Human CEACAM1 (hCEACAM1) is a single pass type I transmembrane protein expressed as 12 alternatively spliced isoforms that all contain an N-terminal V set fold of the immunoglobulin superfamily (IgV) ectodomain followed by up to three type 2 constant immunoglobulin (IgC2) ectodomains (A1, B, A2), a transmembrane sequence, and a signaling cytoplasmic domain. CEACAM1 function is triggered by intercellular or trans binding of the IgV domain, resulting in higher order surface CEACAM1 oligomerization and subsequent intracellular signal transduction. In contrast to other immunoreceptors such as the T cell inhibitory and mucin domain-containing protein 3 (TIM-3), programmed cell death protein 1 (PD-1), and programmed death-ligand 1 (PD-L1), CEACAM1 serves as its own primary ligand, owing to high affinity homophilic interactions of its unique IgV domain, as well as an important microbial receptor. The displaced CC′ loop forms a cleft with the FG loop that exposes the key residues F29, S32, Y34, V39, G41, Q44, Q89, I91, N97, and E99 critical in mediating homophilic CEACAM1 interactions.

The V39A mutant crystal contained two copies of a hCEACAM1 GFCC′ face–mediated homodimer in the asymmetric unit. The first hCEACAM1 V39A dimer comprising molecules (a) and (b) resembled a WT homodimer with RMSD of 0.7 Å (over 1482 atoms), whereas the second GFCC′-mediated dimer comprising molecules (c) and (d) featured important conformational differences across several beta strands and loops with RMSD of 3.0 Å (over 1655 atoms) compared to the WT homodimer. The major distinguishing feature of this second V39A homodimer structure compared to that of the WT was the increased separation between interacting CC′ loops (10.0 Å vs 3.7 Å). Further, we observed a considerable decrease in hydrogen bond and weaker hydrophobic interactions at the GFCC′ face in the V39A homodimer, consistent with a less stable and less interactive GFCC′ face that possibly reflects an hCEACAM1 IgV monomer–dimer exchange transition state. Interestingly for both of the V39A-containing dimers, a considerable metal ion electron density (4.0 σ intensity in the 2Fo–Fc electron density map) was observed at V39A molecule (a) and (c); the density was modeled as nickel (Ni++) that was hexa-coordinated by residues H105 and V106 from three neighboring IgV molecules found in the unit cell and crystallographic symmetry mates. A CSS of 0.0 was calculated for the weak GFCC′-mediated V39A dimer (formed by molecules (c) and (d)) consistent with a monomeric species whereas a CSS score of 1.0 was calculated for molecules (a) and (b) consistent with a dimer and thus suggestive of the possibility of both hCEACAM1 V39A monomers and dimers and furthermore, a rapid monomer–dimer exchange model.

>QLTTESMPFNVAEGKEVLLLVHNLPQQLFGYSWYKGERADGNRQIVGYAIGTQQATPGPANSGRETIYPNASLLIQNVTQNDTGFYTLQVIKSDLVNEEATGQFHVY[4x]>[2x]MSYYHHHHHHLEST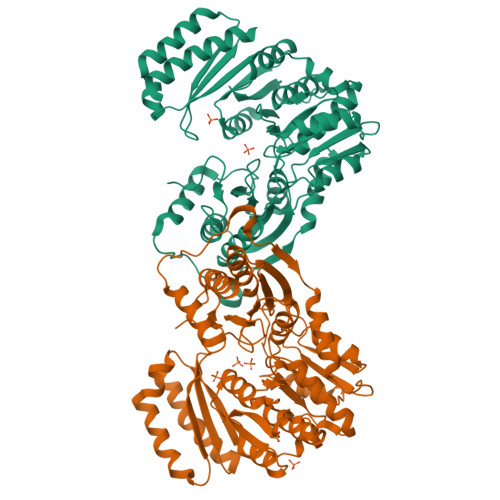SLYKKAGMGKYFGTDGVRGVANKELTPELAFKIGRFGGYVLTKDTDRPKVIIGRDTRISGHMLEGALVAGLLSTGAEVMRLGVISTPGVAYLTKALDAQAGVMISASHNPVQDNGIKFFGSDGFKLTDEQEAEIEALLDKEVDELPRPTGTNLGQVSDYFEGGQKYLQYIKQTVEEDFSGLHIALDCAHGATSSLAPYLFADLEADISTMGTSPNGMNINDGVGSTHPEVLAELVKEKGADIGLAFDGDGDRLIAVDEKGNIVDGDQIMFICAKYMKETGQLKHNTVVSTVMSNLGFYKALEANGITSDKTAVGDRYVMEEMKRGGYNLGGEQSGHIILLDYITTGDGMLSALQLVNIMKMTKKPLSELAGEMTKFPQLLVNVRVTDKKLALENEKIKEIIRVVEEEMNGDGRILVRPSGTEPLIRVMAEAPTQEVCDAYVHRIVEVVKAEVGAE>[4x]MTH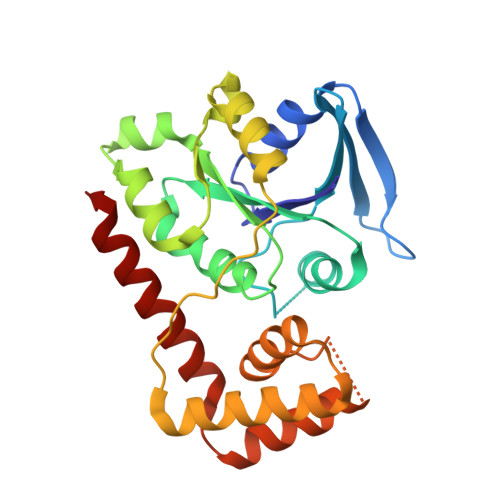ALLIGNPNCGKTTLFNALTNANQRVGNWPGVTVEKKTGEFLLGEHLIEITDLPGVYSLVANAEGISQDEQIAAQSVIDLEYDCIINVIDACHLERHLYLTSQLFELGKPVVVALNMMDIAEHRGISIDTEKLESLLGCSVIPIQAHKNIGIPALQQSLLHCSQKIKPLKLSLSVAAQQILNDLENQLISKGYKNSFAYYFSRRLAEGDTLIGEKAFTESLLIKLQETEQNLDVLLADARYQKIHEIVTLVQKK>[2x]MSLEDGYKVEVGKNAYLPCSYTLPTSGTLVPMCWGKGFCPWSQCTNELLR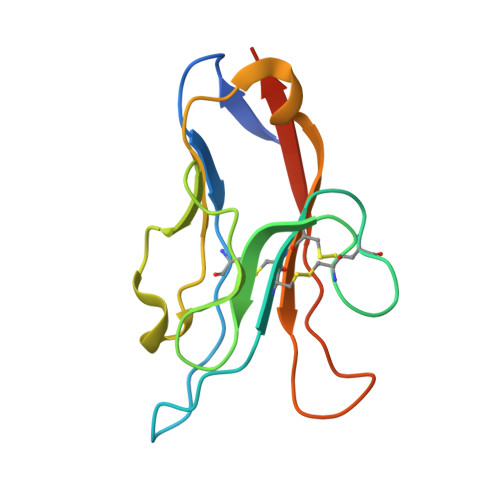TDERNVTYQKSSRYQLKGDLNKGDVSLIIKNVTLDDHGTYCCRIQFPGLMNDKKLELKLDIKAALVPR>[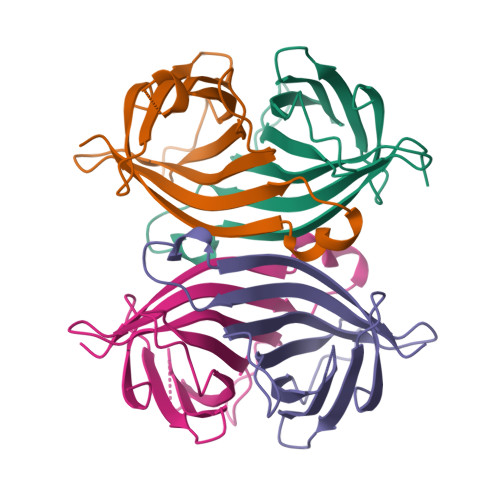4x]AEAGITGTWYNQLGSTFIVTAGADGALTGTYESAVGNAESRYVLTGRYDSAPATDGSGTALGWTVAWKNNYRNAHSATTWSGQYVGGAEARINTQWLLTSGTTEANAAKSTLVGHDTFTKVKPSAAS3-oxo-4-pregnene-20-carboxyl-Coenzyme 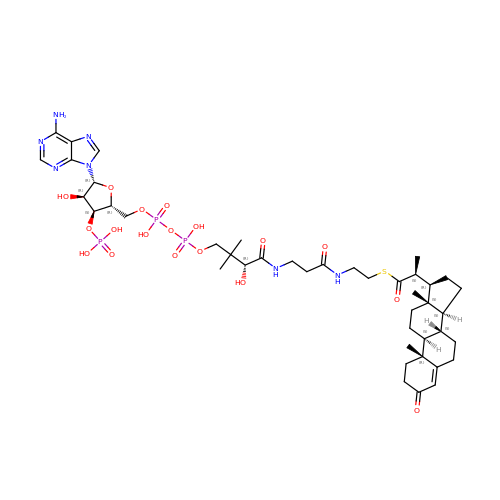A | C43 H66 N7 O18 P3 S | CJJBDUCNUMWUJX-ZKTJOKCMSA-N The bacteriophage T7, Escherichia coli podophage, has been employed as a model for the investigation of the DNA packaging and delivery mechanism among tailed phages and related dsDNA viruses. The tail, connected to a unique vertex of the head by the dodecameric portal gp8, consists of the dodecameric adaptor protein gp11 and the hexameric nozzle protein gp12 (20, 24) surrounded by six trimeric tail fibers gp17 (16, 22, 24). The core is formed by the core proteins gp14, gp15, and gp16; upon virion adsorption onto host membranes or the receptor rough lipopolysaccharide (LPS), these core proteins have been suggested to extend the tail channel and form a trans-envelope channel for genome delivery into the infected cell. In this study, using a 300 kV cryo-electron microscopy (cryo-EM) and defocus refinement with Z-height correction, we provided improved structures of core proteins at a resolution of 3 Å, the portal–tail complex in mature T7 at a resolution of 2.7 Å, and the portal–tail complex in LPS-induced DNA-ejected T7 at a resolution of 3.5 Å.

Through the local reconstruction method and by independently refining the Z-height for different regions, we obtained the structures of the core complex, portal, and portal–tail complex in mature T7 at resolutions of 3, 2.5, and 2.7 Å, respectively. Notably, we identified eight copies of the core protein gp14 and 12 copies of the small protein gp6.7 between the portal barrel and the core, as well as six copies of the small protein gp7.3 at the junction of the adaptor and tail nozzle within the tail channel, which served to anchor the end of the dsDNA. Twelve copies of the gp6.7 loop I, which surrounds the outer surface of the dodecameric portal helical barrel, mediate the interaction between the portal barrel and gp14. We modeled the C-terminal loop (residues 84–98) of 99-residue gp7.3. Six copies of the C-terminal loop, with each copy being anchored to two adjacent nozzle proteins of gp12, are located at the junction of the nozzle and adaptor in the tail channel. Twelve lysine residues (residues K84 and K85) derived from the six copies of gp7.3 interact with the dsDNA end in the portal–tail channel. On the basis of the location of the C-terminus in the resolved structure of gp7.3, the unstructured densities encircling dsDNA can be attributed to the unresolved N-terminus (residues 1–83) in gp7.3. Thus, all gp7.3 molecules interact with both the tail and the DNA end within the portal–tail channel. Our structure revealed that six copies of gp7.3 are located at the junction of the adaptor and nozzle within the tail channel, suggesting that gp7.3 might serve as a structural scaffold to assist the assembly of the nozzle into the adaptor. Additionally, in the tip domain of the mature T7 nozzle, each gp12 molecule contains a three-stranded β-sheet (residues 264–294) with two long hairpins: A (residues 264–282) and B (residues 283–294).

>[12x]MCFSPKIKTPKMDTNQIRAVEPAPLTQEVSSVEFGGSSDETDTEGTEVSGRKGLKVERDDSVAKSKASGNGSARMKSSIRKSAFGGKK;>MGKKVKKAVKKVTKSVKKVVKEGARPVKQVAGGLAGLAGGTGEAQMVEVPQAAAQIVDVPEKEVSTEDEAQTESGRKKARAGGKKSLSVARSSGGGINI[6x];>[18x]MANVIKTVLTYQLDGSNRDFNIPFEYLARKFVVVTLIGVDRKVLTINTDYRFATRTTISLTKAWGPADGYTTIELRRVTSTTDRLVDFTDGSILRAYDLNVAQIQTMHVAEEARDLTTDTIGVNNDGHLDARGRRIVNLANAVDDRDAVPFGQLKTMNQNSWQARNEALQFRNEAETFRNQAEGFKNESSTNATNTKQWRDETKGFRDEAKRFKNTAGQYATSAGNSASAAHQSEVNAENSATASANSAHLAEQQADRAEREADKLENYNGLAGAIDKVDGTNVYWKGNIHANGRLYMTTNGFDCGQYQQFFGGVTNRYSVMEWGDENGWLMYVQRREWTTAIGGNIQLVVNGQIITQGGAMTGQLKLQNGHVLQLESASDKAHYILSKDGNRNNWYIGRGSDNNNDCTFHSYVHGTTLTLKQDYAVVNKHFHVGQAVVATDGNIQGTKWGGKWLDAYLRDSFVAKSKAWTQVWSGSAGGGVSVTVSQDLRFRNIWIKCANNSWNFFRTGPDGIYFIASDGGWLRFQIHSNGLGFKNIADSRSVPNAIMVENE;>MALISQSIKNLKGGISQQPDILRYPDQGSRQVNGWSSETEGLQKRPPLVFLNTLGDNGALGQAPYIHLINRDEHEQYYAVFTGSGIRVFDLSGNEKQVRYPNGSNYIKTANPRNDLRMVTVADYTFIVNRNVVAQKNTKSVNLPNYNPNQDGLINVRGGQYGRELIVHINGKDVAKYKIPDGSQPEHVNNTDAQWLAEELAKQMRTNLSDWTVNVGQGFIHVTAPSGQQIDSFTTKDGYADQLINPVTHYAQSFSKLPPNAPNGYMVKIVGDASKSADQYYVRYDAERKVWTETLGWNTEDQVLWETMPHALVRAADGNFDFKWLEWSPKSCGDVDTNPWPSFVGSSINDVFFFRNRLGFLSGENIILSRTAKYFNFYPASIANLSDDDPIDVAVSTNRIAILKYAVPFSEELLIWSDEAQFVLTASGTLTSKSVELNLTTQFDVQDRARPFGIGRNVYFASPRSSFTSIHRYYAVQDVSSVKNAEDITSHVPNYIPNGVFSICGSGTENFCSVLSHGDPSKIFMYKFLYLNEELRQQSWSHWDFGENVQVLACQSISSDMYVILRNEFNTFLARISFTKNAIDLQGEPYRAFMDMKIRYTIPSGTYNDDTFTTSIHIPTIYGANFGRGKITVLEPDGKITVFEQPTAGWNSDPWLRLSGNLEGRMVYIGFNINFVYEFSKFLIKQTADDGSTSTEDIGRLQLRRAWVNYENSGTFDIYVENQSSNWKYTMAGARLGSNTLRAGRLNLGTGQYRFPVVGNAKFNTVYILSDETTPLNIIGCGWEGNYLRRSSGI[6x];>[12x]MRSYDMNVETAAELSAVNDILASIGEPPVSTLEGDANADAANARRILNKINRQIQSRGWTFNIEEGITLLPDVYSNLIVYSDDYLSLMSTSGQSIYVNRGGYVYDRTSQSDRFDSGITVNIIRLRDYDEMPECFRYWIVTKASRQFNNRFFGAPEVEGVLQEEEDEARRLCMEYEMDYGGYNMLDGDAFTSGLLTR;>[12x]MAEKRTGLAEDGAKSVYERLKNDRAPYETRAQNCAQYTIPSLFPKDSDNASTDYQTPWQAVGARGLNNLASKLMLALFPMQTWMRLTISEYEAKQLLSDPDGLAKVDEGLSMVERIIMNYIESNSYRVTLFEALKQLVVAGNVLLYLPEPEGSNYNPMKLYRLSSYVVQRDAFGNVLQMVTRDQIAFGALPEDIRKAVEGQGGEKKADETIDVYTHIYLDEDSGEYLRYEEVEGMEVQGSDGTYPKEACPYIPIRMVRLDGESYGRSYIEEYLGDLRSLENLQEAIVKMSMISSKVIGLVNPAGITQPRRLTKAQTGDFVTGRPEDISFLQLEKQADFTVAKAVSDAIEARLSFAFMLNSAVQRTGERVTAEEIRYVASELEDTLGGVYSILSQELQLPLVRVLLKQLQATQQIPELPKEAVEPTISTGLEAIGRGQDLDKLERCVTAWAALAPMRDDPDINLAMIKLRIANAIGIDTSGILLTEEQKQQKMAQQSMQMGMDNGAAALAQGMAAQATASPEAMAAAADSVGLQPGI> MPIFRFTALAMTLGLLSAPYNAMAATSNPAFDPKNLMQSEIYHFAQNNPLADFSSDKNSILTLSDKRSIMGNQSLLWKWKGGSSFTLHKKLIVPTDKEASKAWGRSSTPVFSFWLYNEKPIDGYLTIDFGEKLISTSEAQAGFKVKLDFTGWRAVGVSLNNDLENREMTLNATNTSSDGTQDSIGRSLGAKVDSIRFKAPSNVSQGEIYIDRIMFSVDDARYQWSDYQVKTRLSEPEIQFHNVKPQLPVTPENLAAIDLIRQRLINEFVGGEKETNLALEENISKLKSDFDALNIHTLANGGTQGRHLITDKQIIIYQPENLNSQDKQLFDNYVILGNYTTLMFNISRAYVLEKDPTQKAQLKQMYLLMTKHLLDQGFVKGSALVTTHHWGYSSRW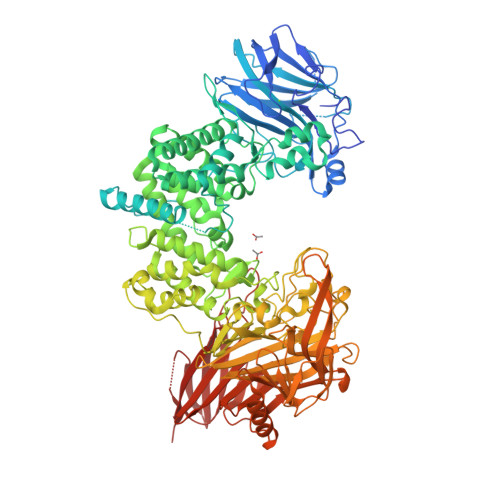WYISTLLMSDALKEANLQTQVYDSLLWYSREFKSSFDMKVSADSSDLDYFNTLSRQHLALLLLEPDDQKRINLVNTFSHYITGALTQVPPGGKDGLRPDGTAWRHEGNYPGYSFPAFKNASQLIYLLRDTPFSVGESGWNNLKKAMVSAWIYSNPEVGLPLAGRHPFNSPSLKSVAQGYYWLAMSAKSSPDKTLASIYLAISDKTQNESTAIFGETITPASLPQGFYAFNGGAFGIHRWQDKMVTLKAYNTNVWSSEIYNKDNRYGRYQSHGVAQIVSNGSQLSQGYQQEGWDWNRMQGATTIHLPLKDLDSPKPHTLMQRGERGFSGTSSLEGQYGMMAFDLIYPANLERFDPNFTAKKSVLAADNHLIFIGSNINSSDKNKNVETTLFQHAITPTLNTLWINGQKIENMPYQTTLQQGDWLIDSNGNGYLITQAEKVNVSRQHQVSAENKNRQPTEGNFSSAWIDHSTRPKDASYEYMVFLDATPEKMGEMAQKFRENNGLYQVLRKDKDVHIILDKLSNVTGYAFYQPASIEDKWIKKVNKPAIVMTHRQKDTLIVSAVTPDLNMTRQKAATPVTINVTINGKWQSADKNSEVKYQVSGDNTELTFTSYFGIPQEIKLSPLP~{N}-[(2~{S})-1-[(3~{R},3~{a}~{R},6~{S},6~{a}~{S})-6-fluoranyl-3-oxidanyl-2,3,3~{a},5,6,6~{a}-hexahydrofuro[3,2-b]pyrrol-4-yl]-4-methyl-1-oxidanylidene-pentan-2-yl]-4-[2-(4-methylpiperazin-1-yl)-1,3-thiazol-4-yl]benzamide 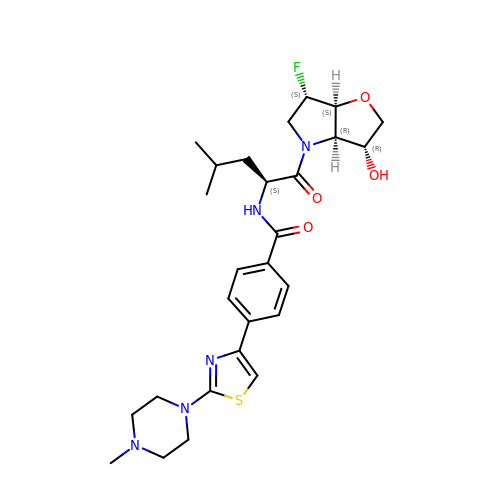| C27 H36 F N5 O4 S | BJRXVCXTMWVZKF-KVFBUXGHSA-N>[2x]GMPKPINVRVTTMDAELEFAIQPNTTGKQLFDQVVKTIGLREVWYFGLHYVDNKGFPTWLKLDKKVSAQEVRKENPLQFKFRAKFYPEDVAEELIQDITQKLFFLQVKEGILSDEIYCPPETAVLLGSYAVQAKFGDYNKEVHKSGYLSSE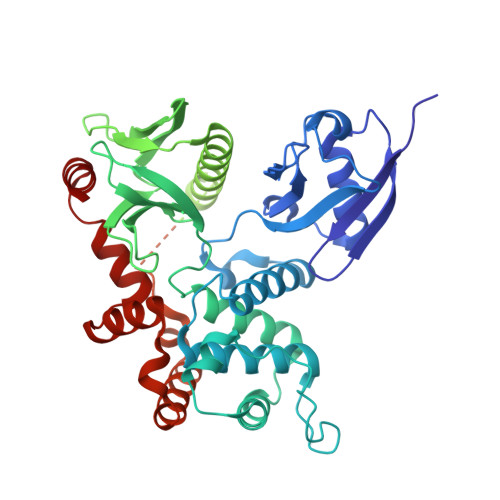RLIPQRVMDQHKLTRDQWEDRIQVWHAEHRGMLKDNAMLEYLKIAQDLEMYGINYFEIKNKKGTDLWLGVDALGLNIYEKDDKLTPKIGFPWSEIRNISFNDKKFVIKPIDKKAPDFVFYAPRLRINKRILQLCMGNHELYMRRRKPDTIEVQQMKAQAREEKHQKQLERQQLETEKKRRETVEREKEQMMREKEELMLRLQDYEEKTKKAERELSEQIQRALQLEEERKRAQEEAERLEADRMAALRAKEELERQAVDQIKSQEQLAAELAEYTAKIALLEEARRRKEDEVEEWQHRAKEAQDDLVKTKEELHLVMTAPPPPPPPVYEPVSYHVQESLQDEGAEPTGYSAELSSEGIRDDRNEEKRITEAEKNERVQRQLLTLSSELSQARDENKRTHNDIIHNENMRQGRDKYKTLRQIRQGNTKQRIDEFEAL> MKHHHHHH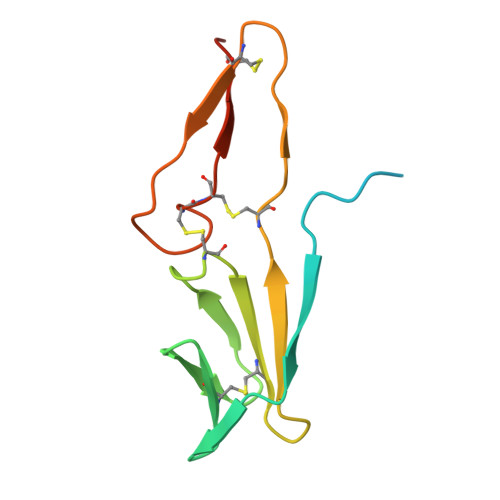SAGLEVLFQGPMGDVQERGHTYVTKNVTVEDGACVYLRNVIPNGETKALNNPCVLSTCYAADRKVNSTLCPNIGVDEGCHVEWTPDGVYPNCCPKHVCPSATASS> SVLRPQLTFEHPVDNSPTPFRPVYYDEKGVRHVGEPGVHPFAERIKAVSVPSEQLLLKTETPYLSLVTCPLTFVDTVEDLEALVAVLLNETEIAVDLEHHDFYSYQGFTCLMQISTRTQDFIVDCLKVRANMYLMAPVFLQPNIVKVFHGAREDVRWLQKDFGLYIVNLFDTSIALQNLHMPHSLAFAVDHFCQVKLNKKYQTADWRVRPIPAEMVSYAQQDTHFLLYVYDRLKQLLLNCEARASVGNMLLHVFQESRLLSLERYEKPHLDPDVTYKQALGRSLGGLSSSQLQVAREIFNWRDMAAREADDSPSAVMHISCVLSIATKLPTSANEVLKCCSPVSVAVRTNVMKLLQIVKDAIGSALEHHHHHH

The exosome is a 3′–5′ exoribonuclease complex that plays a central role in numerous pathways related to RNA processing and degradation, both in the nucleus and in the cytoplasm. The eleventh exosome subunit, RRP6, is a member of the DEDD superfamily (DEDD-Y subgroup) of divalent metal dependent exonucleases. Rrp6 is composed of an N-terminal PMCN2NT domain which was shown to interact with a cofactor Rrp47, the EXO domain containing the catalytic active site, an HRDC (helicase and RNAseD C-terminal) domain, and a C-terminal region responsible for the interaction with the exosome. The EXO domain consists of a classical α/β fold composed by a six-stranded β-sheet flanked by α-helices and the HRDC domain is constituted of six α-helices.

The TbRRP6CAT construct crystallized in a sea urchin-like form composed of very thin needles. TbRRP6CAT crystal structure was refined at 2.4 Å resolution to final Rfactor/Rfree of 16%/22%, respectively. The model covers residues 176 to 541 and includes 185 solvent molecules. The polypeptide chain was clearly defined by the electron density, except the residues 416 to 423 that could not be modeled. TbRRP6CAT shares 41% and 40% of sequence identity with the corresponding catalytic core of the yeast and human proteins respectively and, as expected, conserves their overall architecture. The T. brucei RRP6 structure shows a closer match to the human RRP6, both proteins presenting a shorter linker and a more accessible active site. TbRRP6CAT is the first RRP6 described up to now that was crystallized with the native catalytic site DEDD-Y comprised by the residues D271, E273, D329, D397 and Y393. In the TbRRP6CAT crystal structure, these residues exhibit a configuration similar to the mutated active sites of the human and the yeast structures, even in the absence of metal ions or nucleotides. The apo TbRRP6CAT catalytic site shows only moderate movements of the side chains comparing with Mn/AMP bound Rrp6 structure, and a water molecule that is coordinated by Y393 and E273 residues could represent the hydrolytic water. The electron density map revealed the presence of a disulfide bond between the residues C496 and C515, linking α-helix 3 and the end of α-helix 4 of the HRDC domain.> MNLPTAQEVQGLMARFIELVDVGDIEAIVQMFADDATVEDPFGQPPIHGREQIAAFFRQGLGGGKVR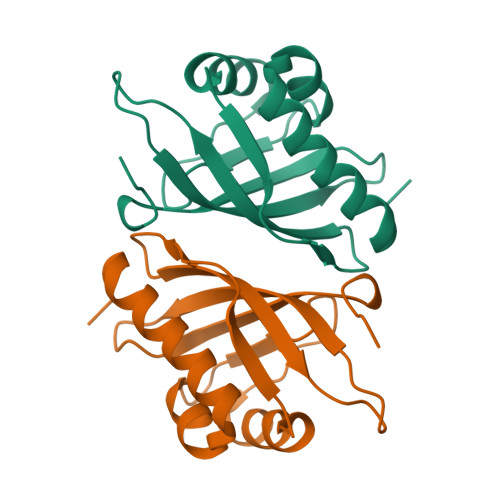ACLTGPVRASHNGCGAMPFRVEMVWNGQPCALDVIDVMRFDEHGRIQTMQAYWSEVNLSVREPQ>GPFTLDHAPRITLRMRSHRVPCGQNTRFILNVQSKPTAEVKWYHNGVELQESSKIHYTNTSGVLTLEILDCHTDDSG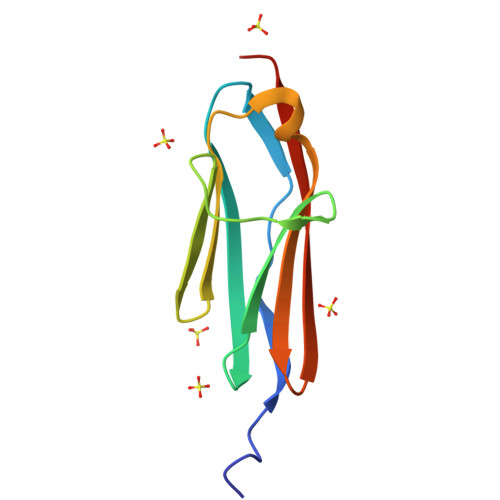TYRAVCTNYKGEASDYATLDVTGGDY[3x]>[4x]MIEKQMDRVVKEMRRQLEMIDKL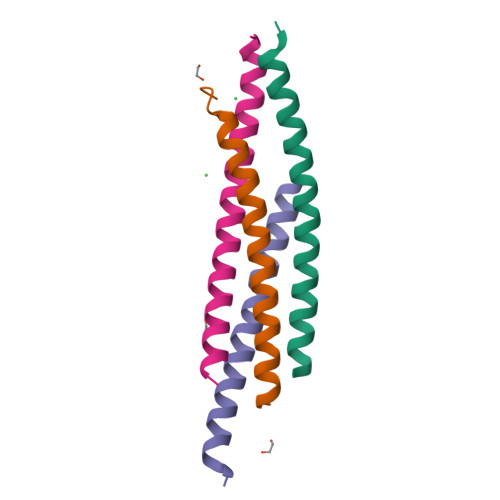TTREIEQVELLKRIHDKLVVQSTGEIDMTK> MTLTYWDKEKRMTLKQMIQQVAINEQENELTHYVFTTPLSMPTFGKPMLGYVPLNEVATSKFFSNVNDFDRDNQLAMAHFPDTTITQAYNLTNSIKPGDTSLPDAEVAALKWFWKFFTSINLVRQPPMDNVMYWACQFLSSGTSFLPLERDVEIVFSGFKGSHICMFSNLRQMNLSPILCPYYDLITNFKTTTEIRAYVDAHEELKSLLTYLCLCTIVGLCDTFTETRNMDTGEYVWKVRDVVSRNHTPAQNVEKFCYTIQNAKYMIQLVHVLLFPLTDNKYADLPNYVAVITQGAINQSRSHNVINTTDESNSNTTSDTAASTSGIVSGDTGTVASLYPDEFKYVQS;>MRPIRMYKNNQERTNLKHQEINEEQQNEQTTSNQGFTRSDNSGKINIERISSSRNQITDGKTVSSYSKIETNRSSQDSVQHGGSSITYTSDTTGNPRITNARTNNDETHATGPIEDLNSTSHGREP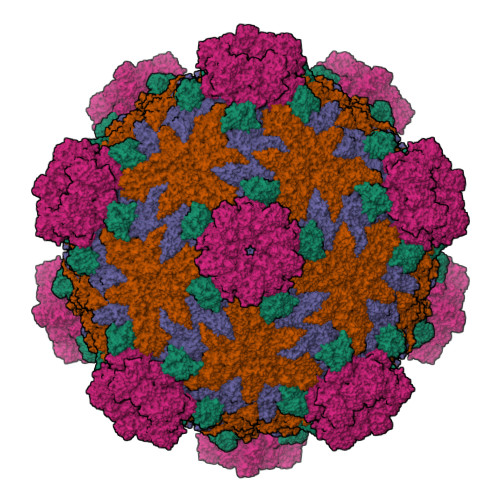EIESFADRAELAMMIQGMTVGALTVQPMRSIRSTFANLANVLIFHDVFTTEDKPSAFIEYHSDEMIVNMPKQTYNPIDNLAKILYLPSLEKFKYGTGIVQLNYSPHISKLYQNTNNIINTITDGITYANRTEFFIRVMVLMMMDRKILTMEFYDVDTSAISNTAILPTIPTTTGVSPLLRIDTRTEPIWYNDAIKTLITNLTIQYGKIKTVLDANAVKRYSVVGYPIDQYRAYLYNHNLLEYLGKKVKREDIMSLIKALSYEFDLITISDLEYQNIPKWFSDNDLSRFIFSICMFPDIVRQFHALNIDYFSQANVFTVKSENAIVKMLNSNQNMEPTIINWFLFRICAIDKTVIDDYFSLEMTPIIMRPKLYDFDMKRGEPVSLLYILELILFSIMFPNVTQHMLGQIQARILYISMYAFRQEYLKFITKFGFYYKIVNGRKEYIQVTNQNERMTENNDVLTGNLYPSLFTDDPTLSAIAPTLAKIARLMKPTTSLTPDDRAIAAKFPRFKDSAHLNPYSSLNIGGRTQHSVTYTRMYDAIEEMFNLILRAFASSFAQRPRAGVTQLKSLLTQLADPLCLALDGHVYHLYNVMANMMQNFIPNTDGQFHSFRACSYAVKDGGNIYRVVQNGDELNESLLIDTAIVWGLLGNTDSSYGNAIGATGTANVPTKVQPVIPTPDNFITPTIHLKTSIDAICSVEGILLLILSRQTTIPGYEDELNKLRTGISQPKVTERQYRRARESIKNMLGSGDYNVAPLHFLLHTEHRSTKLSKPLIRRVLDNVVQPYVANLDPAEFENTPQLIENSNMTRLQIALKMLTGDMDDIVKGLILHKRACAKFDVYETLTIPTDVKTIVLTMQHISTQTQNNMVYYVFLIDGVKILAEDIKNVNFQIDITGIWPEYVITLLLRAINNGFNTYVSMPNILYKPTITADVRQFMNTTKAETLLISNKSIVHEIMFFDNALQPKMSSDTLALSEAVYRTIWNSSIITQRISARGLMNLEDARPPEAKISHQSELDMGKIDETSGEPIYTSGLQKMQSSKVSMANVVLSAGSDVIRQAAIKYNVVRTQEIILFE[2x];> MIDLRLEEDILTATLPEFLSTRPKYRYAYTNTKQQDIRFQGPMRHVRLTHLYKQTKLWNLQYIERELAISEIDDALDEFIQTFSLPYVIEQGTYKYNMLLGMHAHNVNYQDDVSELIANNPQLLNYLDDNPFSAIFELVNVDLQIYQYGQNIFNNEAEHTILFLKDNTNYGVIQALQKHPFSATHINWHLHKHIFVFHSREQLLNKLLSAGLEDSQLYQRQKTYSTKRGDRPTERMVTYIEDDHIRRIQAVFPLLLDNIFDVKLHKDSSMTWLKSYADMIYDSVKNSNSTITPEIRKLYLRMYNQYMRIFLPIEQYMLYDNTCWPFSEKITLKINVRLISSRENQPVLWKTPIDTENLISIVQPDEPINKLNFTAIPSTMIRLNDNITMYRAVKDMFSAIEYLPDAIENIPTLTMKEQALSRYISPDSEAQNFFNNQPPYLNSIMNVNRQVFEAVKRGNIQVSTGSMEHLCLCMHVKSGLIVGRTVLIDDKVVLRRNFNASTAKMITCYVKAFAQLYGEGSLINPGLRMVFFGVETEPAIDILKLFYGDKSLYIQGFGDRGIGRDKFRTKIEDALTLRIGCDILISDIDQADYEDPNEEKFDDITDFVCYVTELVISNATVGLVKISMPTYYIMNKISSTLNNKFSNVAINIVKLSTQKPYTYEAYIMLSHGSTLTNKGYLRNPVCDVYLEKISLQPMDLKIISTISNEINYDKPTLYRFVVDKNDVTDVSIAMHILSIHCSTITTRSVMVRSDNTGAFVTMSGIKDMKRVAIMNRMTDGTSANSYMHEQNGKLYLQKVPYLEDLISAFPNGFGSTYQNDYDSSMSVINVNALIRQVVYRVISKSIPVALLESLSRIRIIGGRDLGEMNAVYKLYKTPIEVYDAVGITREYPHVQISYRAQRYSFTESIPNHTLLLANYVIMNDVDGAPISSLEQINTIKKIISKISLGSIAYIQVYTDIVARNINVMTKNDSFLISANADKTVFKVQVSGYKAVEMCNYEQLLQLVSDNTGVNIIKLTYQDVLESCVLSSGILGDTGSWLLDLVLASTYIIEIRG>[4x]MAVIFHEKTKEFHIFNREVSYLMRIMENGQLENLYYGKVIRDKEDFGYLHEEAMRSQMSVCIPEPGILSMQYTRQEYPVYGTGDYRSPALTVLQENGSRLVDFSYVSHEIYKGKKGIPPLPSTYAESEDEAETLEVTLHDQVTDTDLVLTYTIYEDYPVITRNARFEQKGEQKIVLERAMSASVEFLDMDYELVQLSGAWSRERYVKNRKLEMGIQSVHSLNGTCGGAEHNPFIALKRPQTTENQGEVYGFS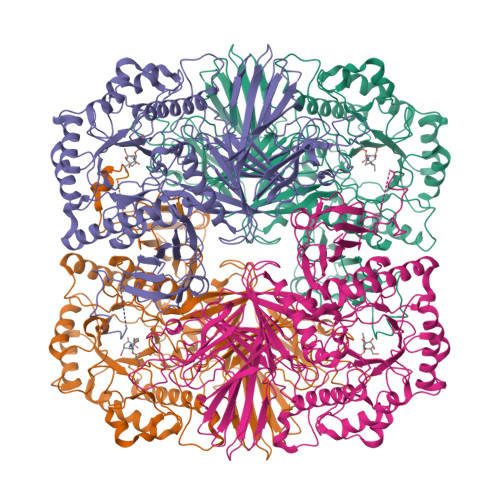LVYSGNFLAQAEVSTFDMTRVMLGINPEDFSWELNQGESFQTPEVVMVYSDRGLNKMSQAYHRLYRTRLMRVTWRDKARPILLNNWEATYFDFNEEKILKIAEKAKEAGVELFVLDDGWFGARNDDYRGLGDWYVNLEKLPDGIAGLSRKVEALGLKFGLWVELEMVNKDSDLYRAHPDWLIGAPDRFESHARHQHVLDFSRKEVVDYIYKMIAKVLRESSISYIKWDMNRYMTEPYSRGADASQQGKVMHKYILGVYDLYTRLTTEFPEILFESCASGGARFDPAMLYFAPQTWTSDDTDASERTKIQYGTSYVYPVVSMGSHVSAVPNHQMHRMTPIETRANVAYFGTFGYELDLNLLSEAELESVKKQIAFMKEYRELIQVDGDFYRLLSPFEGNETAWMVVAQDKSRAVAAFYQRMNKVNASWIRFKLQGLDAGTLYEVSCDMAPSASYDESLAKIYGIQTEENMVKTYRAYGDELMQVGIPIDREDLNKKGGDFASLLYTLKKVTD> PNIIKRSAWE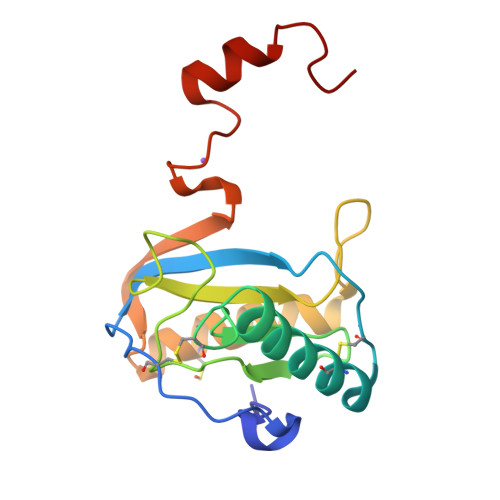ARETHCPKMNLPAKYVIIIHTAGTSCTVSTDCQTVVRNIQSFHMDTRNFCDIGYHFLVGQDGGVYEGVGWHIQGSHTYGFNDIALGIAFIGYFVEKPPNAAALEAAQDLIQCAVVEGYLTPNYLLMGHSDVVNILSPGQALYNIISTWPHFKH M. tuberculosis GpgS catalyzes the formation of glucosyl-phosphoglycerate, using an activated glucose donor and 3-phosphoglycerate. To investigate the structure and specificity of this novel glycosyltransferase family we have solved the crystal structure of M. tuberculosis GpgS, both unliganded and in complex with Mg2+, UDP and 3-phosphoglycerate. The structure of M. tuberculosis GpgS comprises a single globular domain with an overall conical shape, displaying an eight-stranded, predominantly parallel β/α/β sandwich. The structure can be subdivided into two closely associated subdomains, the N-terminal nucleotide binding subdomain (residues 45–137), composed of a four stranded β-sheet (β4, β3, β2, β5) flanked on either side by two α-helices and resembling the Rossmann-like fold, and the C-terminal subdomain (residues 138–281), consisting of a mixture of α/β secondary structure, usually highly variable in GTs with the GT-A fold, and shown to be involved in acceptor substrate recognition.

In order to further understand the nucleotide and sugar specificity of this enzyme family, we have succeeded in obtaining the structure of the GpgS-UDP-phosphoglycerate ternary complex at 2.7 Å resolution and the ligands UDP, 3-phosphoglycerate and Mg2+ could be readily located in the electron density maps. The structure of the ternary complex was refined to a final R-factor of 20.4% (R-free 23.5%), and binding of the nucleotide does not induce gross structural changes in GpgS (overall rmsd 0.28 Å over 279 equivalent Cα atoms). The only significant structural changes occur in the loop connecting strand β8 and helix α9, where large movements of Asn260 and Arg256 are observed. The flexibility of this loop impaired modeling of the Ala257-His258-Arg259 segment in the ternary complex. The occupancy of the UDP and Mg2+ ion in the final structure is below unity, indicating that not all active sites are occupied by these ligands. Consequently, the loop containing residues Ala257-His258-Arg259, as well as residues that are found to interact with the bound nucleotide and probably with the metal ion (see below), might have more than one conformation in the crystals of the ternary complex, thus explaining its apparent disorder upon ligand binding. Although with fractional occupancy in our crystal structure, the electron density clearly indicates that the UDP molecule binds in a hydrophobic cleft located in the Rossmann-like N-terminal subdomain of GpgS. The Mg2+ ion displays axial coordination to the oxygens (O1B and O1A) of the α- and β-phosphate groups and to Asp136 (OD2). In the ternary complex of GpgS the electron density around this region is un-interpretable, probably because in some molecules the His side chain might be facing the coordinated metal and in other it might shift its position by 180°, as observed in the structures of MgS with and without bound nucleotide.

> MTASELVAGDLAGGRAPGALPLDTTWHRPGWTIGELEAAKAGRTISVVLPALNEEATIESVIDSISPLVDGLVDELIVLDSGSTDDTEIRAIASGARVVSREQALPEVPVRPGKGEALWRSLAATSGDIVVFIDSDLINPHPLFVPWLVGPLLTGEGIQLVKSFYRRPLQVSDVTSGVCATGGGRVTELVARPLLAALRPELGCVLQPLSGEYAASRELLTSLPFAPGYGVEIGLLIDTFDRLGLDAIAQVNLGVRAHRNRPLDELGAMSRQVIATLLSRCGIPDSGVGLTQFLPGGPDDSDYTRHTWPVSLVDRPPMKVMRPRKLAAALEHHHHHH> TQEIYPIKEANGRTRKALIICNTEFKHLSLRYGANFDIIGMKGLLEDLGYDVVVKEELTAEGMESEMKDFAALSEHQTSDSTFLVLMSHGT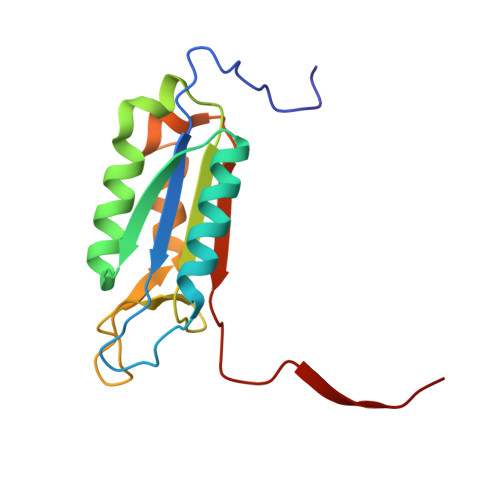LHGICGTMHSEKTPDVLQYDTIYQIFNNCHCPGLRDKPKVIIVQAARGGNSGEMWIRES>[2x]TCGLRQYSQPQFRIKGGLFADIASHPWQAAIFAKHRRSPGERFLCGGILISSCWILSAAHCFQERFPPHHLTVILGRTYRVVPGEEEQKFEVEKYIVHKEFDDDTYDNDIALLQLKSDSSRCAQESSVVRTVCLPPADLQLPDW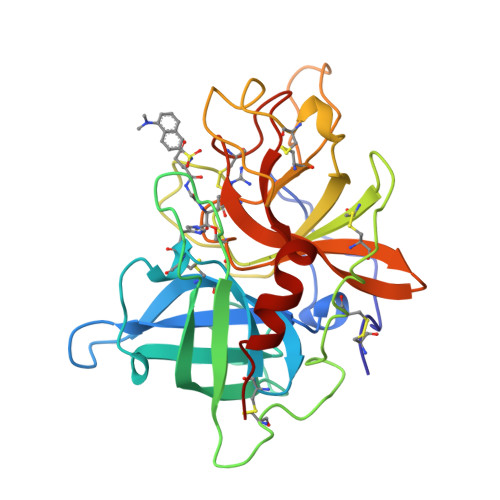TECELSGYGKHEALSPFYSERLKEAHVRLYPSSRCTSQHLLNRTVTDNMLCAGDTRSGGPQANLHDACQGDSGGPLVCLNDGRMTLVGIISWGLGCGQKDVPGVYTKVTNYLDWIRDNMRP>GSHMSLFDFFKNKGSAATATDRLKLILAKERTLNLPYMEEMRKEIIAVIQKYTKSSDIHFKTLDSNQSVET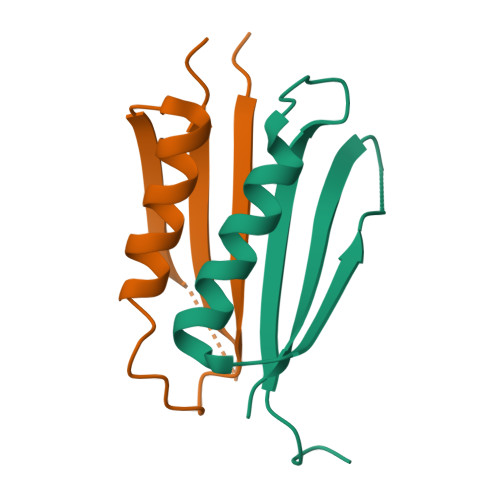IEVEIILPR[2x]>SMSARKRIVVGVAGGIAAYKACTVVRQLTEAGHSVRVVPTESALRFVGAATFEALSGNPVHTGVFTDVHEVQHVRIGQQADLVVIAPATADLLARAVAGRADDLLTATLLTARCPVLFAPAMHTEMWLHPATVDNVATLRRRGAVVLEPASGRLTGADSGPGRLPEAEEITTLAQLLLERADALPYDMAGVKALVTAGGTREPLDPVRFIGNRSSGKQGYAVARVLAQRGADVTLIAGNTAGLIDPAGVEMVHIGSATQLRDAVSKHAPDANVLVMAAAVADFRPAHVAAAKIKKGASEPSSIDLVRNDDVLAGAVRARADGQLPNMRAIVGFAAETGDANGDVLFHARAKLERKGCDLLVVNAVGENRAFEVDHNDGWLLSADGTESALEHGSKTLMATRIVDSIAAFLKS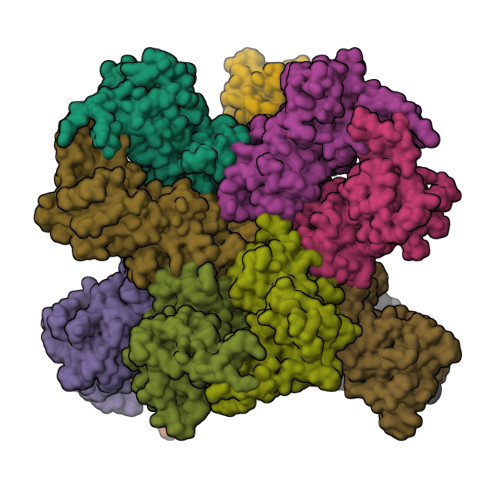QDG[4x]>[2x]MMITLDHVTKQYKSSARPALDDINVKIDKGEFVFLIGPSGSGKSTFMRLLLAAETPTSGDVRVSKFHVNKLRGRHVPKLRQVIGCVFQDFRLLQQKTVYDNVAFALEVIGKRTDAINRVVPEVLETVGLSGKANRLPDELSGGEQQRVAIARAFVNRPLVLLADEPTGNLDPETSRDIMDLLERINRTGTTVLMATHDHHIVDSMRQRVVELSLGRLVRDEQRGVYGMDR;>MRFGFLLNEVLTGFRRNVTMTIAMILTTAISVGLFGGGMLVVRLADSSRAIYLDRVESQVFLTEDVSANDSSCDTTACKALREKIETRSDVKAVRFLNRQQAYDDAIRKFPQFKDVAGKDSFPASFIVKLENPEQHKDFDTAMKGQPGVLDVLNQKELIDRLFAVLDGLSNAAFAVALVQAIGAILLIANMVQVAAYTRRTEIGIMRLVGASRWYTQLPFLVEAMLAATMGVGIAVAGLMVVRALFLENALNQFYQANLIAKVDYADILFITPWLLLLGVAMSGLTAYLTLRLYVRR[2x]

The FtsEX complex is a widely conserved regulator of peptidoglycan (PG) hydrolases. Instead, it functions as a transmembrane signal transduction system for activating PG hydrolases. Briefly, the ATPase activity by the cytoplasmic FtsE powers the system through its ATP cycle, interacting with the transmembrane FtsX. The signal is then transmitted from the cytosolic FtsE to the two extracellular loops of FtsX via conformational changes, and finally to the coiled-coil (CC) domain proteins.

Single-particle Cryo-EM analysis allowed structural determination of the complete WT FtsEX with an overall resolution of 3.9 Å. Cryo-EM density provides a perfect description of the full oligomeric arrangement for the FtsEX system composed by two chains of the cytosolic FtsE NBD domains and two chains of the FtsX with TMD domains inserted into the membrane and the ECD domains protruding to the periplasmic space. Dimerization of the two FtsX protomers occurred through extensive hydrophobic interactions between TM2 and TM3, and the interface between FtsE and FtsX involved a large interacting area of ~960 Å2, contributing to a stable MtbFtsEX complex with a robust ATPase activity. The ECD domains in both FtsX monomers presented a well-defined density. Specifically, while the ECD dimer of other Type VII ABC transporters, such as MacB28, LolC29, and the recently resolved PaeFtsEX8, are oriented with their lower lobes facing each other, the two ECD domains of MtbFtsEX face aside in opposite directions. To understand the structural differences, we compared their structures and found an obvious kink in TM1 of MtbFtsEX, which is absent in other Type VII structures. The kink occurs at the hinge region of TM1 that directly connects to the ECD domain. The kink in TM1 of MtbFtsEX alters the orientation of the coupled ECD domain, resulting in a distinct conformation in which the two ECD hooks with the two lower lobes facing in opposite directions. The binding site for RipC is a large groove in the middle of the ECD domain that is formed when the two lower lobes are positioned on opposite sides away from the central axis of FtsEX.> VANSVLFPCKYASSGCEITLPHTEKADHEELCEFRPYSCPCPGASCKWQGSLDAVMPHLMHQHKSITTLQGEDIVFLATDINLPGAVDWVMMQSCFGFHFMLVLEKQEKYDGHQQFFAIVQLIGTRKQAENFAYRLELNGHRRRLTWEATPRSIHEGIATAIMNSDC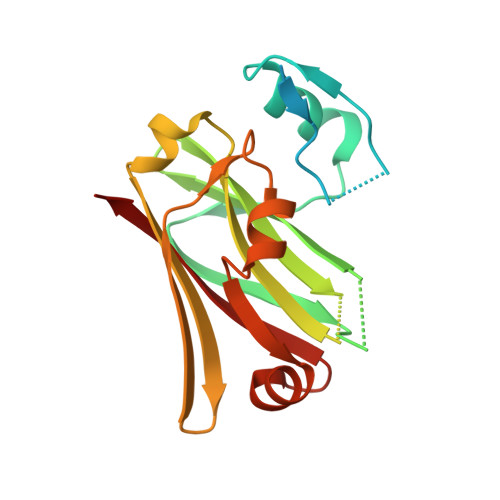LVFDTSIAQLFAENGNLGINVTISMC>[2x]SRKTYTLTDYLKNTYRLKLYSLRWISDHEYLYKQENNILVFNAEYGNSSVFLENSTFDEFGHSINDYSISPDGQFILLEYNYVKQWRHSYTASYDIYDLNKRQLITEERIPNNTQWVTWSPVGHKLAYVWNNDIYVKIEPNLPSYRITWTGKEDIIYNGITDWVYEEEVFSAYSALWWSPNGTFLAYAQFNDTEVPLIEYSFYSDESLQYPKTVRVPYPKAGAVNPTVKFFVVNTDSLSSVTNATSIQITAPASMLIGDHYLCDVTWATQERISLQWLRRIQNYSVMDICDYDESSGRWNCLVARQHIEMSTTGWVGRFRPSEPHFTLDGNSFYKIISNEEGYRHICYFQIDKKDCTFITKGTWEVIGIEALTSDYLYYISNEYKGMPGGRNLYKIQLSDYTKVTCLSCELN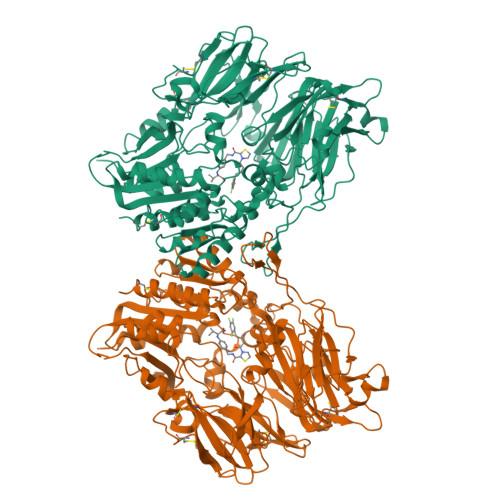PERCQYYSVSFSKEAKYYQLRCSGPGLPLYTLHSSVNDKGLRVLEDNSALDKMLQNVQMPSKKLDFIILNETKFWYQMILPPHFDKSKKYPLLLDVYAGPCSQKADTVFRLNWATYLASTENIIVASFDGRGSGYQGDKIMHAINRRLGTFEVEDQIEAARQFSKMGFVDNKRIAIWGWSYGGYVTSMVLGSGSGVFKCGIAVAPVSRWEYYDSVYTERYMGLPTPEDNLDHYRNSTVMSRAENFKQVEYLLIHGTADDNVHFQQSAQISKALVDVGVDFQAMWYTDEDHGIASSTAHQHIYTHMSHFIKQCFSHHHHHH>[4x]DCCLSVTQKPIPGYI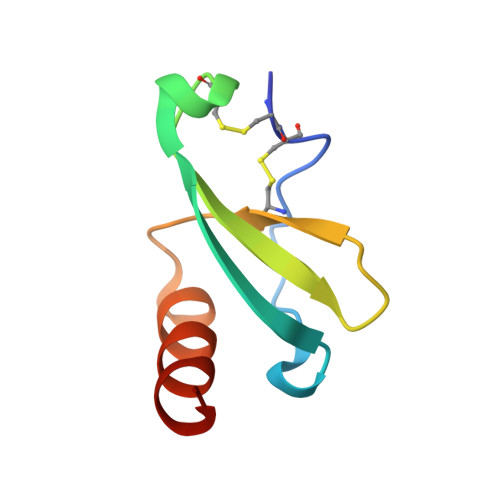VRNFHYLLIKDGCRVPAVVFTTLRGRQLCAPPDQPWVERIIQRLQRTSA> MSTLADQALHNNNVGPIIRA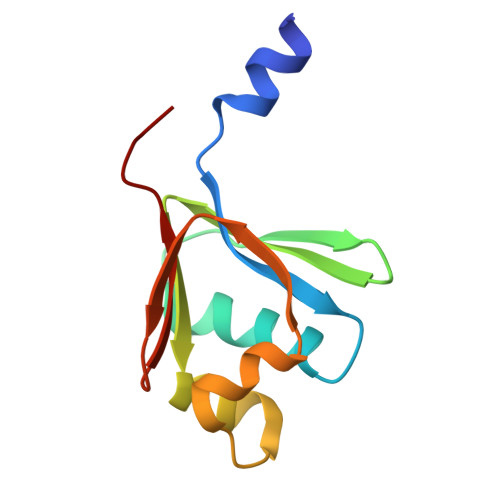GDLVEPVIETAEIDNPGKEITVEDRRAYVRIAAEGELILTRKTLEEQLGRPFNMQELEINLASFAGQIQADEDQIRFYFDKTM> YSTEVEAA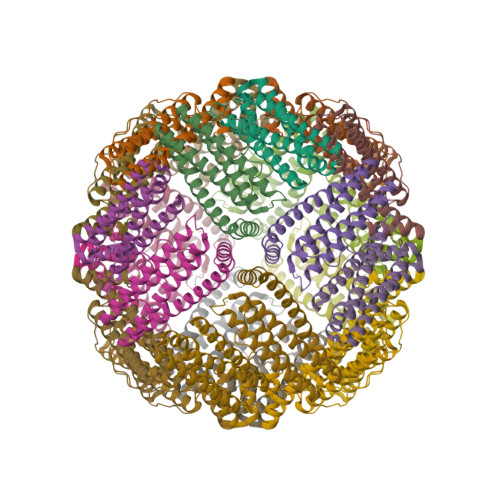VNRLVNLYLRASYTYLSLGFYFDRDDVALEGVCHFFRELAEEKREGAERLLKMQNQRGGRALFQDLQKPSQDEWGTTPDAMKAAIVLEKSLNQALLDLHALGSAQADPHLCDFLESHFLDEEVKLIKKMGDHLTNIQRLVGSQAGLGEYLFERLTLKHD> GRNGK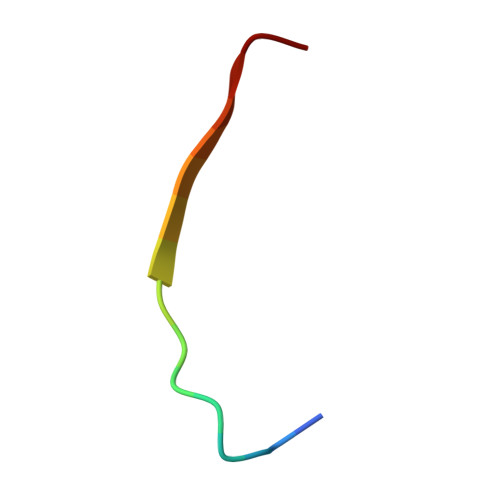SQSIIVGPWGD3-(thiophen-2-ylsulfanylmethyl)benzoic acid | C12 H10 O2 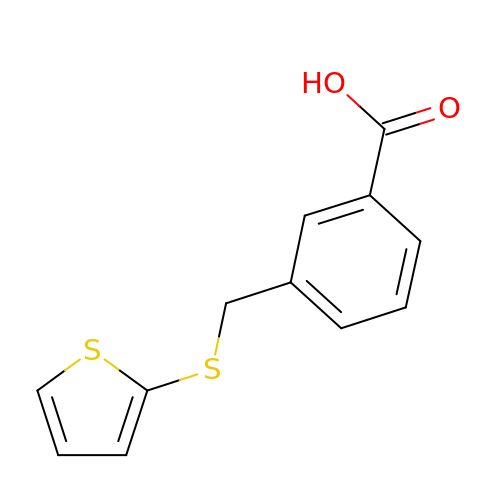S2 | WSMPZJFCOIZVQR-UHFFFAOYSA-N> IDPVLEYRLSQVQSRISEERFLKNNGSGNEIGFWIFDYPAQNELQVREHLKYLLRNLEKDHKFAHLNIFQIIVDMLTERGLFDRVCQQEVKVGTEALKKQLVGLLNQKKIADYIAKKVDLQNQEFVILTGMGNAWPLVRGHELMSALQDVMGFTPLLMFYPGTYSGHDLSPLAGIDSRNYYRAFRLVPESGPAATLNPR;> MTLQNQEFIAGLKAKFAEHRIVFWHDPDKRFLEELDNLELENVTLLDMTDQSQLAVKKRIEIDEPEQQFLLWFPHDAPPKEFDWLLDIRLYSTEFHADFAAITLNTLGIPQLGLREHIQRRKAFFSTKRLSALKGLVTEQENEASLDKKMVAVIAGVKTAKTEEILFSLITQYVNQQKDDDSDLENTLAMLKRHDLEGVLWDILNQEMGYQAEHPTLENLILKLFCTDLSAQADPQKREWLEKNVLATPSGRASALAFMVTWRADRRYKEAYDYCAQQMQDALRPEDQYRLSSPYDLHECETTLSIEQTIIHALVTQLLEESTTLDREAFKKLLSERQSKYWCQTRQEYCAIYDALRQAERLLNLRNRHIDGFHYQDSATFWKAYCEELFRFDQAYRLFNEYALLVHSKGAMILKSLDDYIEALYSNWYLAELSRSWNKVLETENRMQEWRIAGVPRQQNFYNEVVKPQFNNPQIKRVFVIISDALRYEVAEELGNQINTE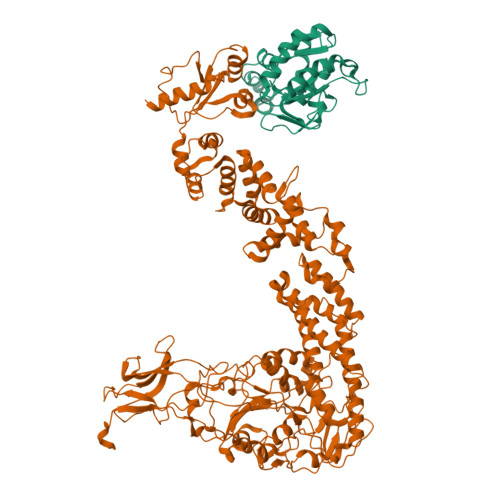KRFTAELRSQLGVLPSYTQLGMAALLPHDEICYQPGSGDIVYADGLSTSGTPNRDTILKKYKGMAVKSDDLLKWKNQQGRDLIRDYEVVYIWHNTIDAMGDSASTEEKTFEACRNAVVELKDLVTRVINRLHGTRIIVTADHGFLFQQQPLSGQDKTTLQIKPDNTIKNHKRFIIGHQLPADDFCWKGKVADTAGVSDNSEFLIPKGIQRFHFSGGARFVHGGAMLQEVCVPVLQVKALQKTAAEKQPQRRPVDIVKHHPLIKLVNNIDKVSLLQTHPVGELYEPRTLNIFIVDNANNVVSGKERICFDSDNNTMEKRVRDVTLKLIGANFNRRNEYWLILEDAQTETGYQKYPVIIDLAFQDDFFKETAAAKFERQHMDSSTSAA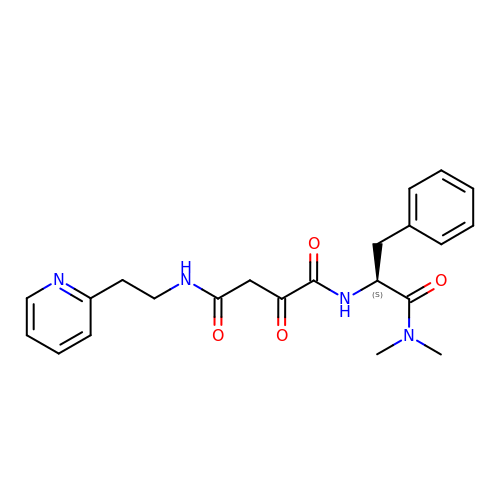N1-(1-DIMETHYLCARBAMOYL-2-PHENYL-ETHYL)-2-OXO-N4-(2-PYRIDIN-2-YL-ETHYL)-SUCCINAMIDE | C22 H26 N4 O4 | ZPFPZRVOBBMZMP-SFHVURJKSA-N>DWPVYHRIDGPIVMIGFGSIGRGTLPLIERHFAFDRSKLVVIDPSDEARKLAEARGVRFIQQAVTRDNYRELLVPLLTAGPGQGFCVNLSVDTSSLDIMELARENGALYIDTVVEPWLGFYFDPDLKPEARSNYALRETVLAARRNKPGGTTAVSCCGANPGMVSWFVKQALVNLAADLGVTGEEPTTREEWARLAMDLGVKGIHIAERDTQRASFPKPFDVFVNTWSVEGFVSEGLQPAELGWGTFERWMPDNARGHDSGCGAGIYLLQPGANTRVRSWTPTAMAQYGFLVTHNESISIADFLTVRDAAGQAVYRPTCHYAYHPCNDAVLSLHEMFGSGKRQSDWRILDETEIVDGIDELGVLLYGHGKNAYWYGSQLSIEETRRIAPDQNATGLQVSSAVLAGMVWALENPNAGIVEADDLDFRRCLEVQTPYLGPVVGVYTDWTPLAGRPGLFPEDIDTSDPWQFRNVLVR[2x]

In contrast to its eukaryotic counterparts, bacterial HSS synthesizes 1 mol HSP from 2 mol PUT. NAD+ serves as a non-covalently bound prosthetic group for BvHSS. The interface area of the dimer was calculated as approximately 1700 Å2 by PDBsum indicating a stable dimer23. The BvHSS subunit consists of two domains as determined by CATH24: one “NAD(P)-binding Rossmann-like” domain (domain 1, residues 3–163 and 394–425) and one “homospermidine-synthase-like domain” (domain 2, residues 164–395 and 426–477) as shown in Fig. 2a and S1. The crystal structures of BvHSS containing NAD+ clearly show that the active site is localized inside each subunit.

The pocket is a “boot-shaped” cavity that is approximately 21 Å deep. The entry to the pocket is formed by part of the “track-and-trace” loop (residues Phe-122 to Asp-125) and the α-helix J at the protein surface. The active site is situated between residues Asn-162, Trp-229, Glu-237, His-296, and the nicotine amide ring of NAD+ at the narrow end of the pocket. Residues Val-115, Val-116, Tyr-123, Asn-135, Leu-138, Pro-163, Gln-240, Thr-295, and Asn-297 form a side pocket at the “heel” of the “boot-shaped” binding pocket, which is filled with six ordered water molecules of which five occur in a nearly planar and equidistant five-membered ring. At least five amino acids (Val-93, Glu-117, Tyr-123, Gly-233, and Ser-236) form a pore at the binding pocket entrance. Narrowing might occur by the bending of the “track-and-trace” loop resulting in a slight rotation of the side chain of Tyr-123 deeper into the pocket and towards Glu-117, accompanied by a side chain rotation of Ser-236 towards the pocket entrance. Thus, the ellipsoid-shaped pore is narrowed from an approximately 4.0 Å times 5.0 Å opening to an approximately 3.3 Å times 3.5 Å opening. Slightly different relative orientations of subunit A to subunit B were observed for all BvHSS structures.>MAPTWFYNTTNSEKLRELQHVLGGSAKLGYLTAKVTEILDVDLETVIRAKAIAAYRAVRVPVIVEHGALCIDALNGLPGALVKPFWESLDTRLCEVIPAGQRTARARGALCYCDGRERHVLIEETEGEIAPSARGTGGFHWDPIFIPKGQTRTFAEMSLDEKLSFSPLGRLHTRLRTELGL[4x];>MTTLTLSEAAPLLKKEFREGRLIPFLGAGFSKPLKLPDGSQLIASLAKTLGFEPELFDMHGRFEQLAEFFAISAPNRLQRLVYEMSLSFDSAEAEALREKSPMHRALAALDWRTIYTTNYDKHVEGALRDAGKQAAVLASFADFQGPRARDVCEVIKFHGTLDQPDTIVLTESSYFQRMALDAPPDQRLRADLLANSFLFIGYSFSDTNIRYIWYRMNQLREQSQLGVKHSQARRCFFATHGAGLVQPDILQQ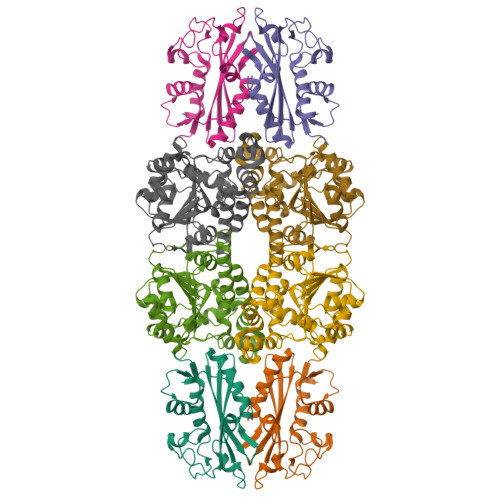WNIDVIQLDPTDKSASVARLLESIA[4x]N-(3-phenylpropyl)adenosine | C19 H23 N5 O4 | 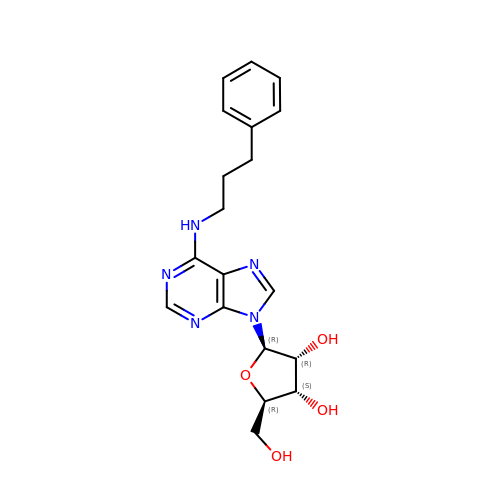UBRRRMDHTZACMR-NVQRDWNXSA-N> MGPAFEFAVAMMKRNSSTVKTEYGEFTMLGIYDRWAVLPRHAKPGPTILMNDQEVGVLDAKELVDKDGTNLELT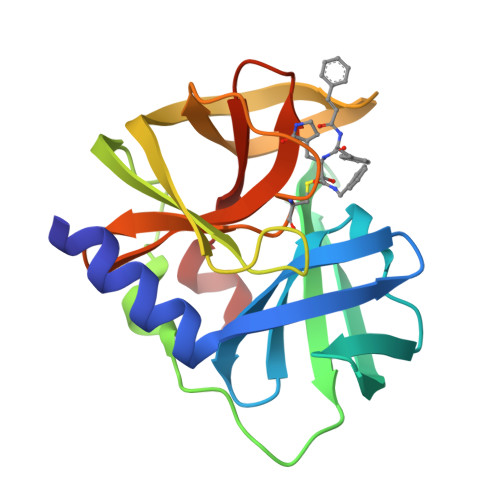LLKLNRNEKFRDIRGFLAKEEVEVNEAVLAINTSKFPNMYIPVGQVTEYGFLNLGGTPTKRMLMYNFPTRAGQCGGVLMSTGKVLGIHVGGNGHQGFSAALLKHYFNDEQ> ADGRSTRYWDCCKPSCGWAKKAPVNQPVFSCNANFQRITDFDAKSGCEPGGVAYSCADQTPWAVNDDFALGFAATSIAGSNEAGWCCACYELTFTSGPVAGKKMVVQSTSTGGDLGSNHFDLNIPGGGVGIFDGCTPQFGGLPGQRYGGISSRNECDRFPDALKPGCYWRFDW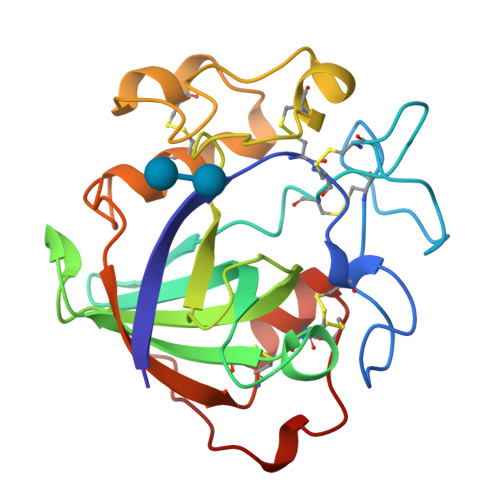FKNADNPSFSFRQVQCPAELVARTGCRRNDDGNFPAVQIP> MYEAVIGLEVHLHLKTRTKMFCGCRADYFGAEPNTHTCPVCLGLPGALPVPNRVAVEHGLRLALALGAEVPERLVFHRKNYFYPDLPKNYQISQYDLPLGRGGSLPLGERRVRIKRLHLEEDAGKSLHLEGRTLLDLNRAGSPLIELVTEPDLKTPEEARLFLQRIQALVQTLGISDASPEEGKLRADVNVSVRRVG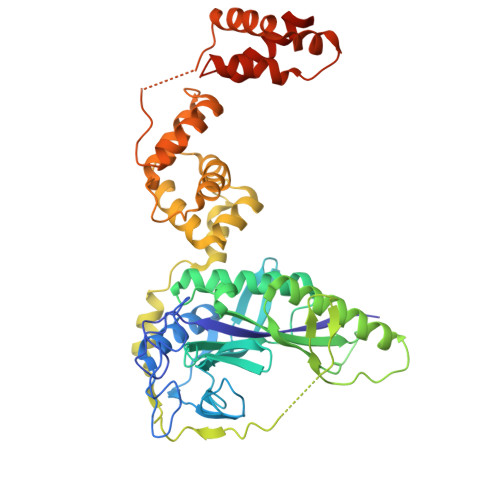EPLGTKVEIKNLNSFKSVQRALEYEIRRQTEILRRGEKVKQATMGFEEGSGKTYPMRTKEEEADYRYFPEPDLPPVAIPRDWLEEVRRSLPELPWEKEARYRALGIKEKDAEVLAYTPSLARFLDQALPLGLASPQALANWLLADVAGLLHERGLRLEETRLSPEGLARLVGLFERGEVTSRVAKSLLPEVLEGQDPEAXXXXXXXXXXXXXXXXXXXXXXXXXXXXXXXXXXXXXXXXXXXXXXXXXXXXXXXXXXXXXXXXXXXXXX> MLYLTQRLEIPAAATASVTLPIDVRVKSRVKVTLNDGRDAGLLLPRGLLLRGGDVLSNEEGTDFVQVIAADEEVSVVRCDDPFMLAKACYALGNRHVPLQI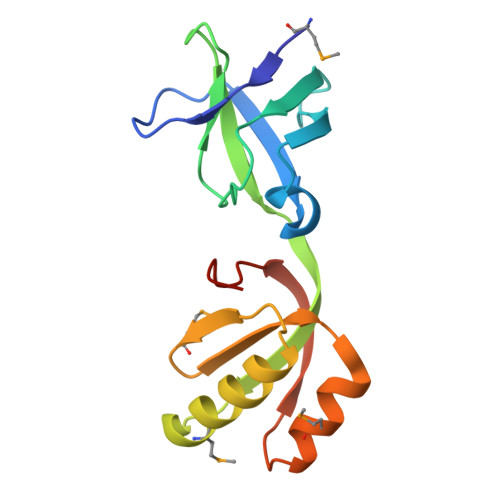MPGELRYHHDHVLDDMLRQFGLTVTFGQLPFEPEAGAYASES>GGCUCUGGAGAGAACCGUUUAAUCGGUCGCCGAAGGAGCA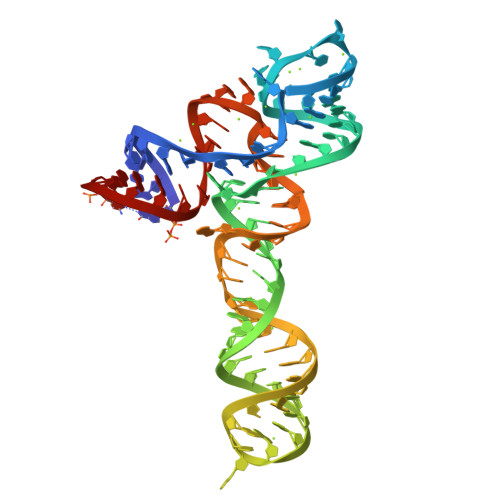AGCUCUGCGGAAACGCAGAGUGAAACUCCCAGGCAAAAGGACAGAGUC[2x]> GPGSDNKEQTGQPLAKDKVALLIGNMSYWEHPKLKAPLVDVYELTNLLRQLDFKVVSLLDLTEYEMCNAVDEFLLLLDKGVYGLLYYAGHGYENFGNSFMVPVDAPNPYRSENCLCVQNILKLMQEKETGLNVFLLDMCRKRNDYDDTIPILDALKVTANIVFGYATCQGAEAFEIQHSGLANGIFMKFLKDRLLEDKKITVLLDEVAEDMGKCHLTKGRQALEIRSSLSEKRALTDPVQGAPCSAEALVRNLQWAKAHELPESMCLKFQCGVHIQLGFAAEFSNVMIIYTSIVHKPPEIIMCDAYVTDFPLDLDIDPKHANKGTPEETGSYLVSKDLPKHCLYTRLSSLQKLKEHLIFTVCLSYQYSGLEDTVEEKQEVNVGKPLIAK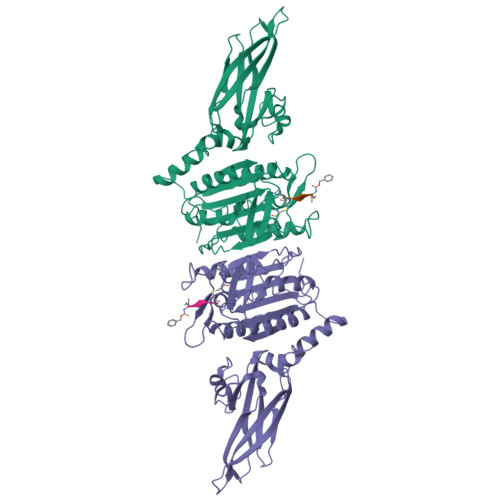LDMHRGL> MMLRTLTRSSAVAGQAVRLFKTSAAAAEGNSVAGIIKSVNETSGANLLSSLKTIKAQAAPIYPAAASST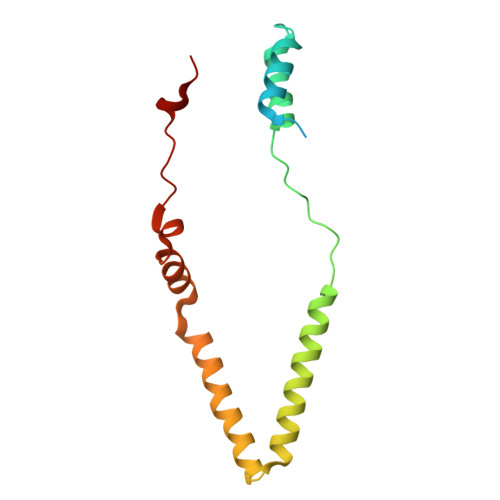GYSTQAKIALFGALSWILYRADGQSKAHEWIVDLNLNVLQAAWLISFSSLIPFRAVYFAFRGMAPATASTLNGLKTFSSISL> MELALRGGYRERSNQDDPEYLEMAHYATSTWSAQQPGKTHFDTVVEVMKVETQTVAGTNYRLTLKVAESTCELTSTYNKDTCQANANAAQRTCTTVIYRNMQGEKSINSFECAA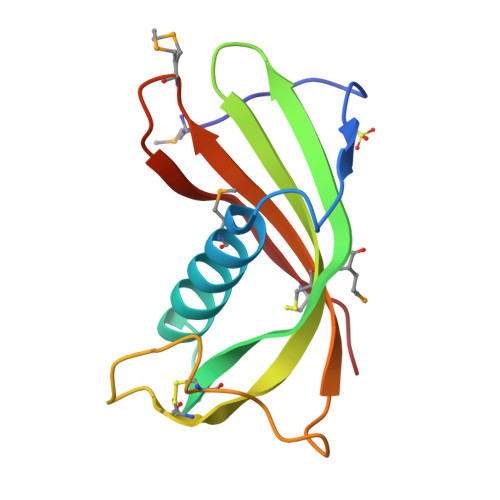A>[6x]MAKNNAVAGFNALNGVELNLFTTDELKAIHYATMEVLMDPGIQVSDPEARQIFKENGCEVNEKTNVVKIPEYLVRKALQLAPSRFVLWGRDKKFNTVQECGGKVHWTCFGTGVKVCKYQDGKYVTVDSVEKDIADIAKLCDWAENIDYFSLPVSARDIAGQGAQDVHETLTPLANTAKHFHHIDPVGENVEYYRDIVKAYYGGDEEEARKKPIFSMLLCPTSPLELSVNACQVIIKGARFGIPVNVLSMAMSGGSSPVYLAGTLVTHNAEVLSGIVLAQLTVPGAKVWYGSSTTTFDLKKGTAPVGSPELGLISAAVAKLAQFYGLPSYVAGSKSDAKVPDDQAGHEKTMTTLLPALAGANTIYGAGMLELGMTFSMEQLVIDNDIFSMVKKAMQGIPVSEETLAVESIQKVGIGNNFLALKQTRQLVDYPSNPMLLDRHMFGDWAAAGSKDLATVAHEKVEDVLKNHQVTPIDADIFKDMQAIVDKADKAFRGMGGHHHHHH

The 22nd genetically encoded amino acid, pyrrolysine, plays a unique role in the key step in the growth of methanogens on mono-, di-, and tri-methylamines by activating the methyl group of these substrates for transfer to a corrinoid cofactor. A substrate:corrinoid methyltransferase catalyzes the demethylation of the specific methylamine, and subsequently transfers this methyl group onto an associated corrinoid protein. In summary, we have determined the structures of native MttB, and its complexes with a substrate analog, sulfite, and its physiological relevant corrinoid protein, MttC. These structures have provided new insights into the mechanism of activation of pyrrolysine that is distinct from the previously determined MtmB structure, and details of the key steps in the pyrrolysine-mediated transfer of methyl groups from methylamine substrates to the cobalamin cobalt in corrinoid proteins.

In our first structure of a pyrrolysine-containing protein, the monomethylamine methyltransferase MtmB, we demonstrated that addition of dithionite to MtmB crystals resulted in addition of a sulfite group to the pyrrolysine imine carbon. We sought to use a similar approach to clarify the details of the conformational states of pyrrolysine in MttB and to provide a structure of this protein bound to a substrate analog. Thus, a MttB crystal was soaked with dithionite and the structure of the resulting MttB-sulfite complex was determined to 3.2 Å resolution. As expected, addition of sulfite to the pyrrolysine imine carbon of MttB was observed with only one strong peak for the sulfite sulfur consistent with a single pyrroline conformation. While the structures of MttB and the MttB-sulfite complex are nearly the same (RMSD = 0.458 and 0.492 Å for the A subunits and overall hexamer, respectively), one significant change was the loss of the water that hydrogen bonds the pyrroline nitrogen in the native MttB structure. It should be noted that the water that hydrogen bonds the pyrroline imine nitrogen in the native MttB structure is absent in both the sulfite-bond MttB and the MttB-MttC complex. This may suggest that during turnover, addition of TMA to pyrrolysine may precede MttC binding—since nucleophilic addition to pyrrolysine would be slower without a hydrogen bond donor.> MKNVGDLMQRLQKMMPAHIKPAFKTGEELLAWQKEQGAIRSAALERENRAMKMQRTFNRSGIRPLHQNCSFENY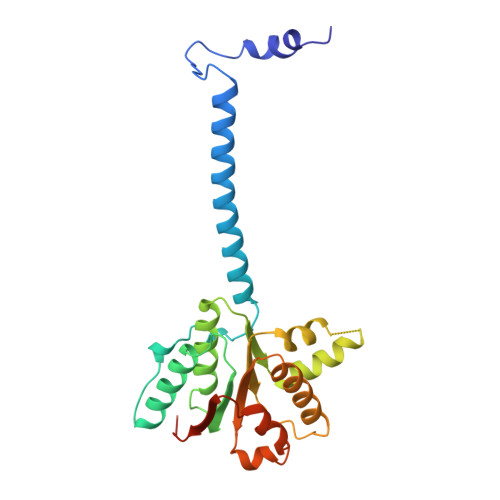RVECEGQMNALSKARQYVEEFDGNIASFIFSGKPGTGKNHLAAAICNELLLRGKSVLIITVADIMSAMKDTFRNSGTSEEQLLNDLSNVDLLVIDEIGVQTESKYEKVIINQIVDRRSSSKRPTGMLTNSNMEEMTKLLGERVMDRMRLGNSLWVIFNWDSYRSRVTGKEY>MGHHHHHHMLHLLEQIRAYCETCWEWQEAHEPGMDQDKNPMPAPVEHQICPAVCVLMK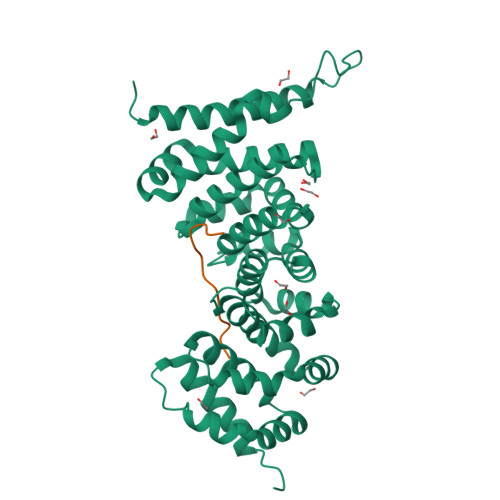LSFDEEHRHAMNELGGLQAIAELLQVDCEMYGLTNDHYSITLRRYAGMALTNLTFGDVANKATLCSMKGCMRALVAQLKSESEDLQQVIASVLRNLSWRADVNSKKTLREVGSVKALMECALEVKKESTLKSVLSALWNLSAHCTENKADICAVDGALAFLVGTLTYRSQTNTLAIIESGGGILRNVSSLIATNEDHRQILRENNCLQTLLQHLKSHSLTIVSNACGTLWNLSARNPKDQEALWDMGAVSMLKNLIHSKHKMIAMGSAAALRNLMANRPAKYKDANIMSPGSSLPS[6x];>PRDSYSGDALYEF[6x]>[4x]MKGFAMLGINKLGWIEKERPVAGSYDAIVRPLAVSP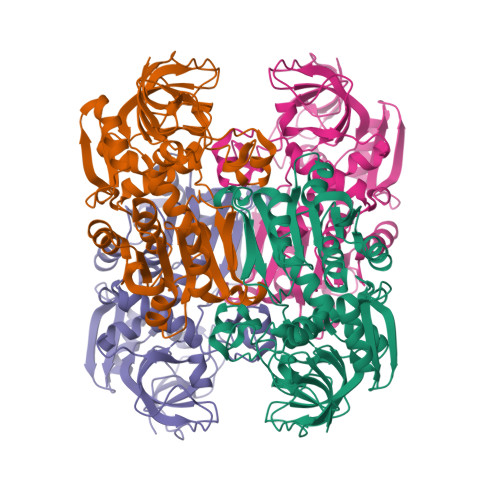CTSDIHTVFEGALGDRKNMILGHEAVGEVVEVGSEVKDFKPGDRVIVPCTTPDWRSLEVQAGFQQHSNGMLAGWKFSNFKDGVFGEYFHVNDADMNLAILPKDMPLENAVMITDMMTTGFHGAELADIEMGSSVVVIGIGAVGLMGIAGAKLRGAGRIIGVGSRPICVEAAKFYGATDILNYKNGHIEDQVMKLTNGKGVDRVIMAGGGSETLSQAVKMVKPGGIISNINYHGSGDALLIPRVEWGCGMAHKTIKGGLCPGGRLRAERLRDMVVYNRVDLSKLVTHVYHGFDHIEEALLLMKDKPKDLIKAVVIL>HHHHHHASLHLLPSPTPNLEIKYTKIFINNEWQNSESGRVFPVYNPATGEQVCEVQEADKADIDKAVQAARLAFSLGSVWRRMDASERGRLLDKLADLVERDRAVLATMESLNGGKPFLQAFYVDLQGVIKTFRYYAGWADKIHGMTIPVDGDYFTFTRHEPIGVCGQIIPWNFPLLMFAWKIAPALCCGNTVVIKPAEQTPLSALYMGALIKEAGFPPGVINILPGYGPTAGAAIASHIGIDKIAFTGSTEVGKLIQEAAGRSNLKRVTLELGGKSPNIIFADADLDYAVEQAHQGVFFNQGQCCTAGSRIFVEESIYEEFVRRSVERAKRRVVGSPFDPTTEQGPQIDKKQYNKILELIQSGVAEGAKLEC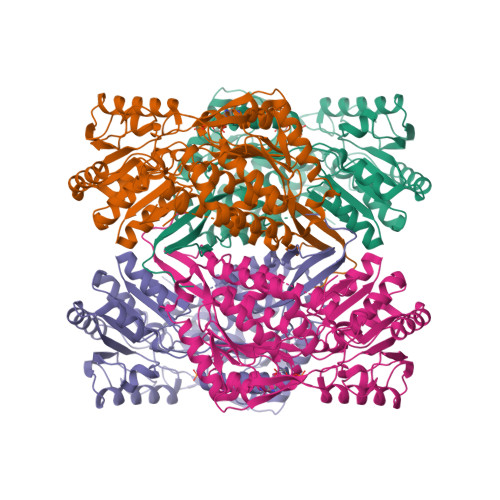GGKGLGRKGFFIEPTVFSNVTDDMRIAKEEIFGPVQEILRFKTMDEVIERANNSDFGLVAAVFTNDINKALTVSSAMQAGTVWINCYNALNAQSPFGGFKMSGNGREMGEFGLREYSEVKTVTVKIPQKNS[4x]> MPSKKKKYNARFPPARIKKIMQTDEEIGKVAAAVPVIISRALELFLESLLKKACQVTQSRNAKTMTTSHLKQCIELEGDPAANKARKEAELAAATAEQ;> GPHMASSSGNDDDLTIPRAAINKMIKETLPNVRVANDARELVVNCCTEFIHLISSEANEICNKSEKKTISPEHVIQALESLGFGSYISEVKEVLQECKTVALKRRKASSRLENLGIPEEELLRQQQELFAKARQQQAELAQQEWLQMQQAAQQAQLAAASASASNQAGSSQDEEDDDDI;> GSHMSGIVPQLQNIVSTVNLGCKL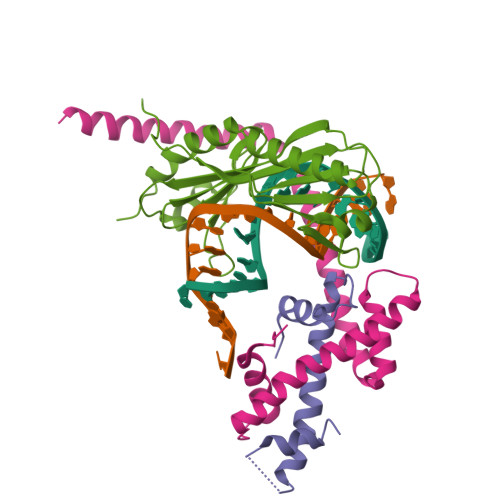DLKTIALRARNAEYNPKRFAAVIMRIREPRTTALIFSSGKMVCTGAKSEEQSRLAARKYARVVQKLGFPAKFLDFKIQNMVGSCDVKFPIRLEGLVLTHQQFSSYEPELFPGLIYRMIKPRIVLLIFVSGKVVLTGAKVRAEIYEAFENIYPILKGFRKTT> MGYYDIDDVLAD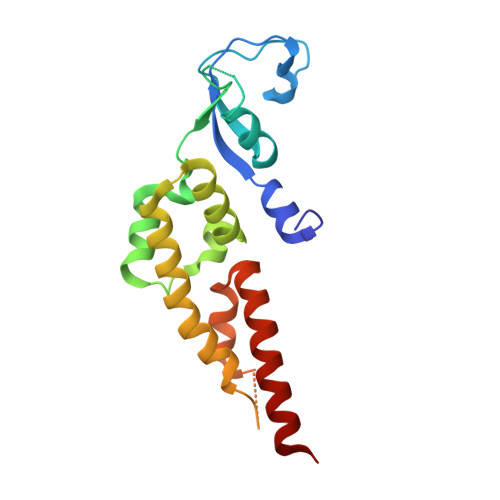GTEFPCKFQYDIPGLGYLENNPGRPITKNTKLNLPLWLARILAIVGGDEALVDEEPVPFVELLPPDMFSTKVMNAIKTDPVALDLHSINSHFFSLAIKWIMLFSEKELANVVSELLLQRAQELNHHASSLSIDLNADSTGKNSANTNIATSTFLLKLEEMEKEIYKKSHESYKDTKRWMFKK>[2x]MSKRPNFLVIVADDLGFSDIGAFGGEIATPNLDALAIAGLRLTDFHTASTASPTRSMLLTGTDHHIAGIGTMAEALTPELEGKPGYEGHLNERVVALPELLREAGYQTLMAGKWHLGLKPEQTPHARGFERSFSLLPGAANHYGFEPPYDESTPRILKGTPALYVEDERYLDTLPEGFYSSDAFGDKLLQYLKERDQSRPFFAYLPFSAPHWPLQAPREIVEKYRGRYDAGPEALRQERLARLKELGLVEADVEAHPVLALTREWEALEDEERAKSARAMEVYAAMVERMDWNIGRVVDYLRRQGELDNTFVLFMSDNGAEGAL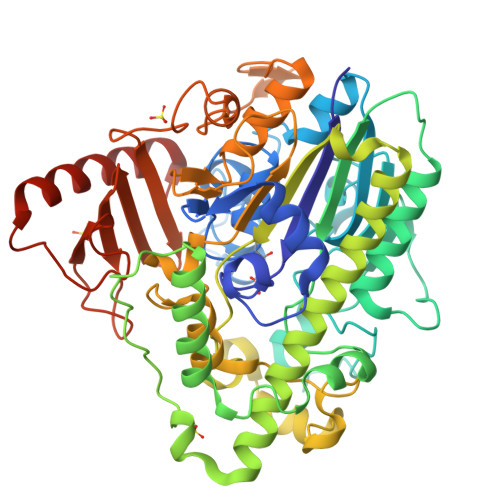LEAFPKFGPDLLGFLDRHYDNSLENIGRANSYVWYGPRWAQAATAPSRLYKAFTTQGGIRVPALVRYPRLSRQGAISHAFATVMDVTPTLLDLAGVRHPGKRWRGREIAEPRGRSWLGWLSGETEAAHDENTVTGWELFGMRAIRQGDWKAVYLPAPVGPATWQLYDLARDPGEIHDLADSQPGKLAELIEHWKRYVSETGVVEGASPFLVR>[2x]SDIHELFVPENKLDHVRAEAETLPSLSITKLD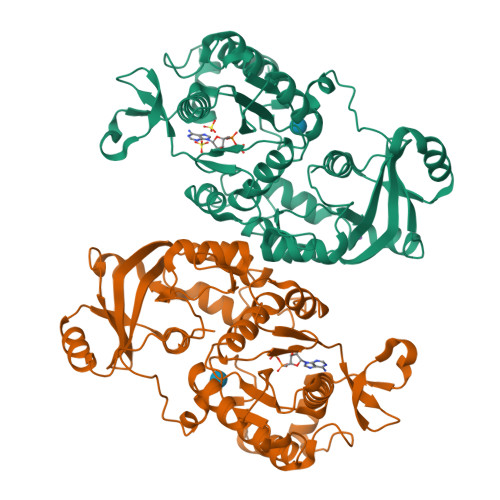LQWVQVLSEGWATPLKGFMREKEYLQVMHFDTLLDDGVINMSIPIVLPVSAEDKTRLEGCSKFVLAHGGRRVAILRDAEFYEHRKEERCSRVWGTTCTKHPHIKMVMESGDWLVGGDLQVLEKIRWNDGLDQYRLTPLELKQKCKEMNADAVFAFQLRNPVHNGHALLMQDTRRRLLERGYKHPVLLLHPLGGWTKDDDVPLDWRMKQHAAVLEEGVLDPKSTIVAIFPSPMLYAGPTEVQWHCRSRMIAGANFYIVGRDPAGMPHPETKKDLYEPTHGGKVLSMAPGLTSVEIIPFRVAAYNKAKKAMDFYDPARHNEFDFISGTRMRKLAREGENPPDGFMAPKAWKVLTDYYRSLEKN>AIELSTDLINKFKDM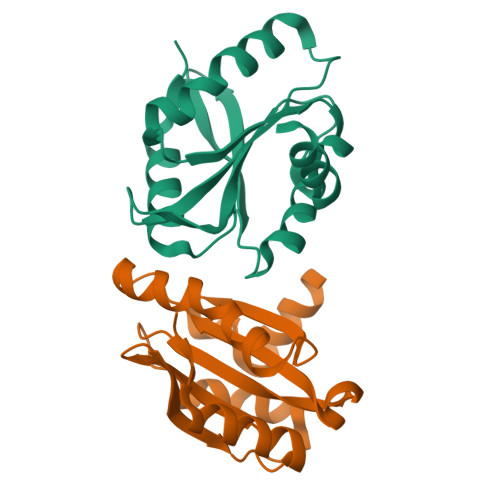NSSGNGRFIQATIVDETINIKAIEQGTSDFDADLDLVLKYLVEGEPSYILFRTETRDDITNGYKWLLLAYIPDRAKVRMKMLYSSTKARFRTTLGGSTFLYEIHGTVFSDFGKSGYEAFLRHE[2x]Type IV pili (T4P)1 are long, surface-exposed filaments which extend from the surfaces of bacterial cells. T4P are composed of both major and minor pilin components, although major pilins comprise the majority of the pilin subunits within each fibre. We identified a cluster of type IV pilin-like genes within the T. thermophilus HB8 genome, using the program PilFind. Three of the remaining six, TTHA1218, TTHA1219 and TTHA1222, yielded crystals of truncated forms which enabled us to solve their structures (designated here as Tt121836-123, Tt121933-236 and Tt122238-123).

Tt122238-123 adopts a typical pilin-like fold, with a central α-helix packed against a 4-stranded antiparallel β-sheet. There is a trimer in the asymmetric unit, with two Tt122238-123 molecules (chains A and B) aligned approximately parallel and a third (chain C) bound in the opposite orientation. Analysis of crystallographic packing by PISA highlighted the interaction between chains A and B as significantly larger than other interfaces, with a buried surface area of 600 Å2, 10 inter-chain hydrogen bonds, 4 salt bridges and a Complexation Significance Score (CSS) score of 0.4. Chain A is transformed onto B by a rotation of 138° and translation of 16.5 Å, possibly indicative of an interaction preserved in fibre assembly. However, such an inference should be treated with caution, given that we observed Tt122238-123 to be monomeric by size exclusion chromatography (SEC; not shown). Given the potential involvement of Tt122238-123 in natural competence, it is interesting that a closely related structure, as judged by r.m.s.d. after superposition, was ComP from N. meningitidis. The ComP fold is more extensive than Tt122238-123, with an additional β-strand (β5) and a loop which wraps around the back of the β-sheet (shown in red in Fig2e). Tt122238-123 therefore appears to lack a specific structural feature, the DD region, necessary for recognition of DNA. Furthermore, calculation of electrostatic surfaces for Tt122238-123 did not reveal a distribution of positive charge which would be characteristic of nucleic acid binding, as noted for ComP. The modeling indicated that the structure of Tt122238-123 could be incorporated into the pilus fibre model, although some repacking of the core helices would be required to satisfy steric constraints (not shown).

>[3x]MANLAAGQSYVRNVALALEAQRDPSTGALPTHLTDCLSGFGQRPKTVTACTITYLNALDYVIEASLDGAALKKVVYKSSDGTLTSLPLEHHHHHH> PPPMAG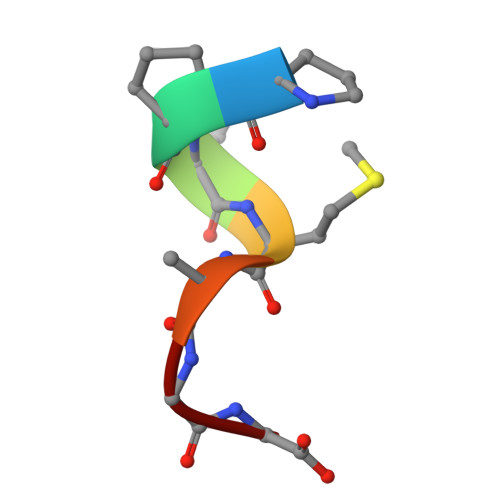G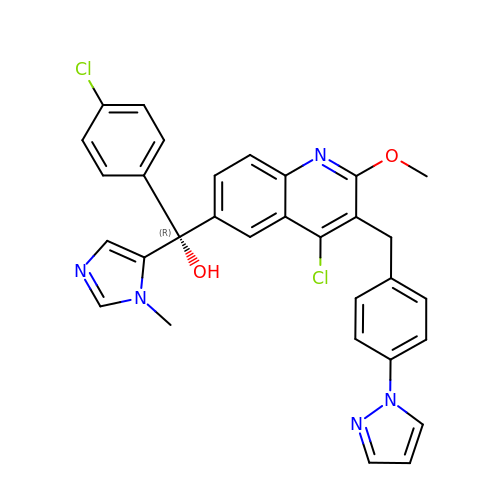(R)-(4-chloro-2-methoxy-3-{[4-(1H-pyrazol-1-yl)phenyl]methyl}quinolin-6-yl)(4-chlorophenyl)(1-methyl-1H-imidazol-5-yl)methanol | C31 H25 Cl2 N5 O2 | UWOBQISTECYGOP-WJOKGBTCSA-N>MYDWFSEMRKKDPVYYDGNIWQVLSYRYTKEVLNNFSKFSSDLTGYHERLEDLRNGKIRFDIPTRYTMLTSDPPLHDELRSMSADIFSPQKLQTLETFIRETTRSLLDSIDPREDDIVKKLAVPLPIIVISKILGLPIEDKEKFKEWSDLVAFRLGKPGEIFELGKKYLELIGYVKDHLNSGTEVVSRVVNSNLSDIEKLGYIILLLIAGNETTTNLISNSVIDFTRFNLWQRIREENLYLKAIEEALRYSPPVMRTVRKTKERVKLGDQTIEEGEYVRVWIASANRDEEVFHDGEKFIPDRNPNPHLSFGSGIHLCLGAPLARLEARIAIEEFSKRFRHIEILDTEKVPNEVLNGYKRLV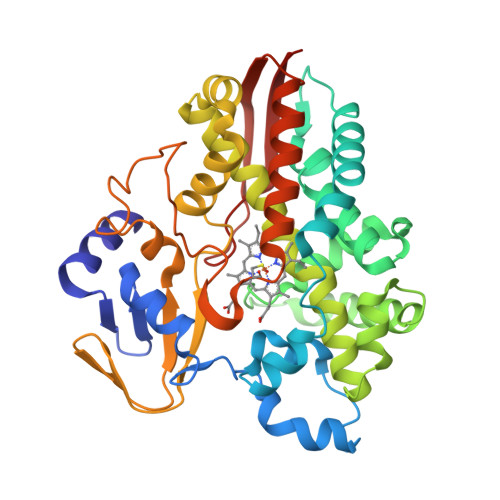VRLKSNE[2x]>[2x]MNIHEWQSKQLIQKYGGRAQSGEVAFSPERSRDIA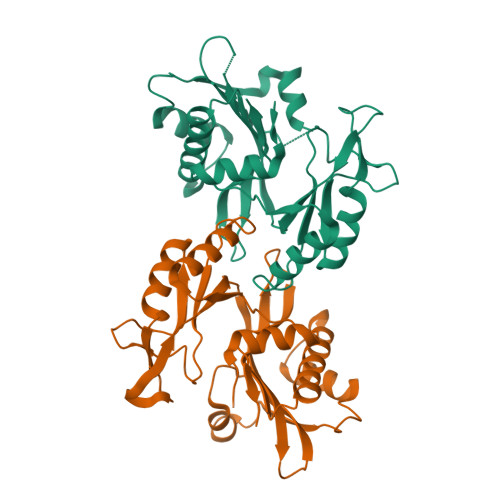KKLWNQFPGCEFVVKAQVLAGGRGKGHWEHGMQGGVKLAKTPEEVYEIANEMIGHKLITKQTGAKGINCNKVMVCGAVDILKEFYLSILLDRAMGCPVIIATSQGGMGIEEVAQKCPECLFKVPISVKNGPTNEQLVKLAKDLGLEGDLVQDCVDNVKALYQVFDKCDSTMVEINPLGVIETPTDEKVICCLDAKIAFDKDAAFGLEHHHHHHHH> GNSKKHNLILIGAPGSGKGTQCEFIKKEYGLAHLSTGDMLREAIKNGTKIGLEAKSIIESGNFVGDEIVLGLVKEKFDLGVCVNGFVLDGFPRTIPQAEGLAKILSEIGDSLTSVIYFEIDDSEII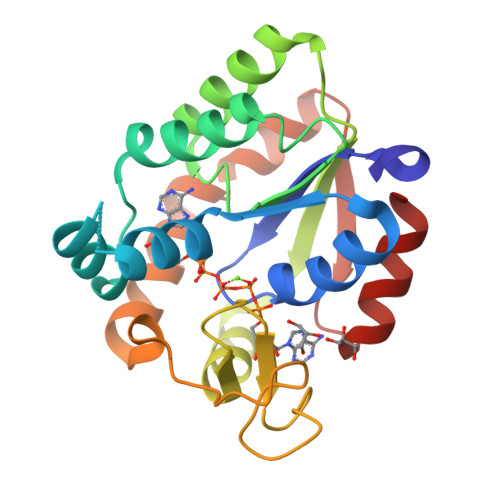ERISGRCTHPASGRIYHVKYNPPKQPGIDDVTGEPLVWRDDDNAEAVKVRLDVFHKQTAPLVKFYEDLGILKRVNAKLPPKEVTEQIKKIL> MARELEGKVAAVTGAASGIGLASAEAMLAAGARVVMVDRDEAALKALCNKHGDTVIPLVVDLLDPEDCATLLPRVLEKACQLDILHANAGTYVGGDLVDADTMAIDRMLNLNVNVVMKNVHDVLPHMIERRTGDIIVTSSLAAHFPTPWEPVYASSKWAINCFVQTVRRQVFKHGIRVGSISPGPVVSALLADWPPE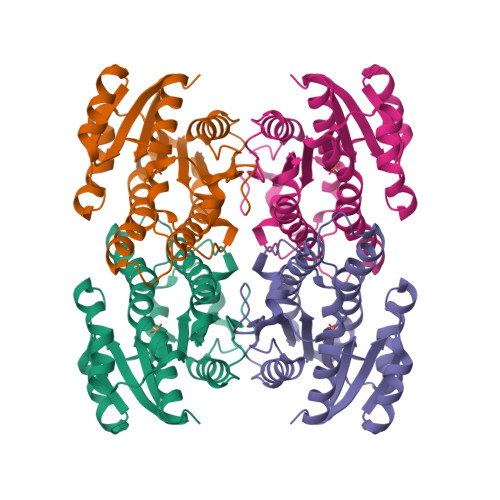KLKEARDSGSLLEASDVAEVVMFMLTRPRGMTIRDVLMLPTNFDL> MIARDPPQEGRLPDPSRL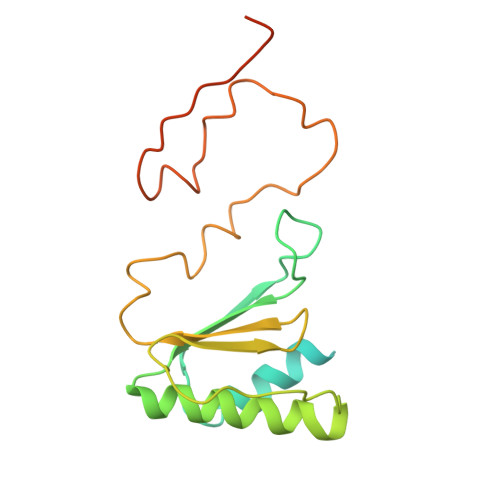PYDDERFAEMLLEMEVNGVIDETWQDAKKARMEDVKEIANILSSLKVRDLCCVDVSEKTSNFDYMMFGTCEGARHIHLAAWAVQDADKVHRISKIKRQQTDELWEVVPVGRIVVNLMVESFREEMTLERKWAVTRSMDPLAAANAPISEGRQVKAHGLWTLTLNLQDLEDFEVDYCKDILMRQM> MDETDPILTQKNWDGTATYFQSSDEHGFSMYYKPQVGFVGDPMPFYDPVAKDFKVMYLQDYRPNPEATYHPIFGVATKDGATYESLGELISCGGRDEQDAAIGTGGTIYNPADKLYYTFYTGNKFKPSSDQNAQVVMVATSPDFKTWTKNRTFYLKGDTYGYDKNDFRDPFLFQTEDGVYHMLIATRKNGKGHIAEFTSADLKEWESAGTFMTMMWDRFYECPDVFK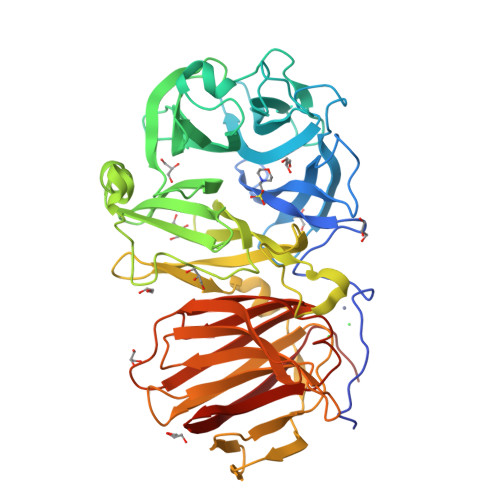MGDWWYLIYSEQASFMRKVQYFKGRTLEDLKATTANDAGIWPDNREGMLDSRAFYAGKTASDGTNRYIWGWCPTRAGNDNGNVGDVEPEWAGNLVAQRLIQHEDGTLTLGVPDAIDRKYTSAQEVKVMAKDGNMIESGKTYTLGEGASVIFNRLKVHNKISFTVKTASNTDRFGISFVRGTDSASWYSIHVNADEGKANFEKDGDDAKYLFDNKFNIPADNEYRVTIYSDQSVCVTYINDQLSFTNRIYQMQKNPWSLCCYKGEITVSDVQVSTYHHHHHH> MVVSKMNKDAQMRAAINQKLIETGERERLKELLRAKLIECGWKDQLKAHCKEVIKEKGLEHV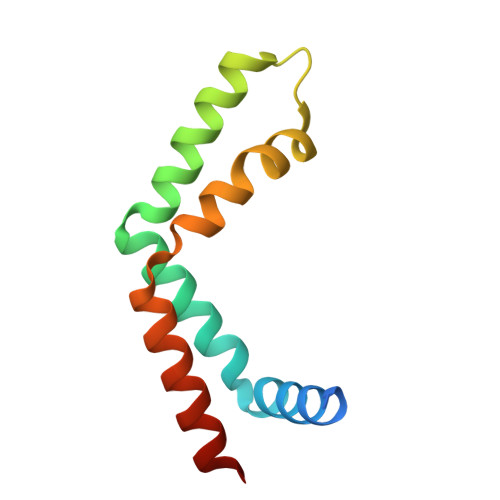TVDDLVAEITPKGRALVPDSVKKELLQRIRTFLAQHASL PYROPHOSPHATE 2- | H2 O7 P2 | 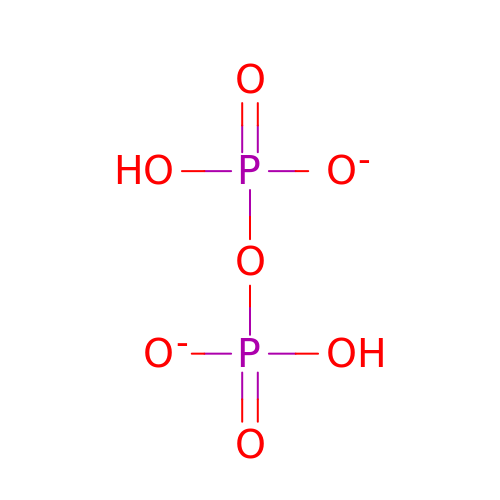XPPKVPWEQAFLFU-UHFFFAOYSA-L>MSKPPPKPVKPGQVKVFRALYTFEPRTPDELYIEEGDIIYITDMSDTNWWKGTSKGRTGLIPSNYVAEQAESIDNPLHEAAKRGNLSWLRECLDNRVGVNGLDKAGSTALYWACHGGHKDIVEMLFTQPNIELNQQNKLGDTALHAAAWKGYADIVQLLLAKGARTDLRNIEKKLAFDMATNAACASLLKKKQGTDAVRTLSNAEDYLDDEDSDLEHHHH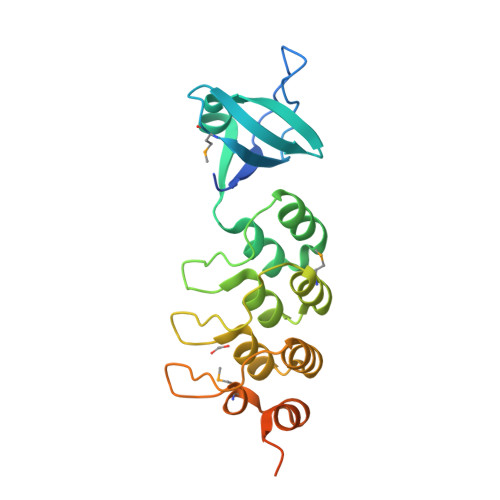HH[2x]> GRSDAYTQVDNFLHAYARGGDELVNGHPSYTVDQAAEQILREQASWQKAPGDSVLTLSYSFLTKPNDFFNTPWKYVSDIYSLGKFSAFSAQQQAQAKLSLQSWSDVTNIHFVDAGQGDQGDLTFGNFSSSVGGAAFAFLPDVPDALKGQSWYLINSSYSANVNPANGNYGRQTLTHEIGHTLGLSHPGDYNAGEGDPTYADATYAEDTRAYSVMSYWEEQNTGQDFKGAYSSAPLLDDIAAIQKLYGANLTTRTGDTVYGFNSNTERDFYSATSSSSKLVFSVWDAGG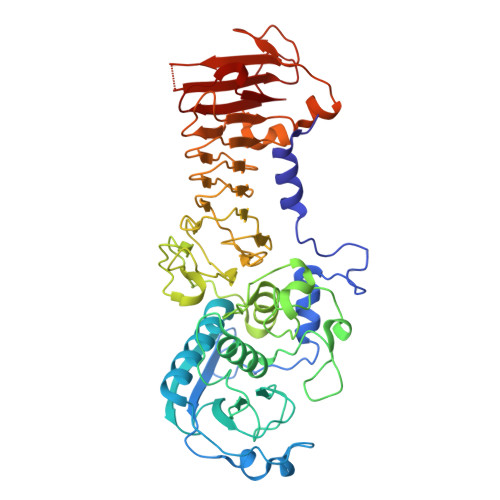NDTLDFSGFSQNQKINLNEKALSDVGGLKGNVSIAAGVTVENAIGGSGSDLLIGNDVANVLKGGAGNDILYGGLGADQLWGGAGADTFVYGDIAESSAAAPDTLRDFVSGQDKIDLSGLDAFVNGGLVLQYVDAFAGKAGQAILSYDAASKAGSLAIDFSGDAHADFAINLIGQATQADIVV5-fluoranyl-3-[[(1~{S},2~{S})-2-phenylcyclopropyl]carbonylamino]-1~{H}-indole-2-carboxylic 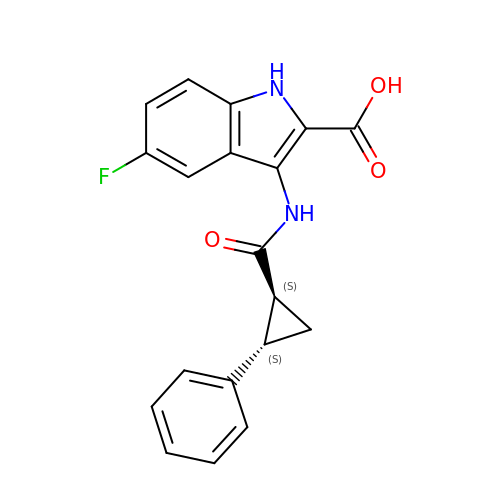acid | C19 H15 F N2 O3 | LBCNHUJFDVBZDB-OLZOCXBDSA-N>GSHMSQATSQPINFQVQKDGSSEKSAMDDYMQHPGKVIKQNNKYYFQTVLNNASFWKEYKFYNANNQELATTVVNDNKKADTRTINVAVEPGYKSLTT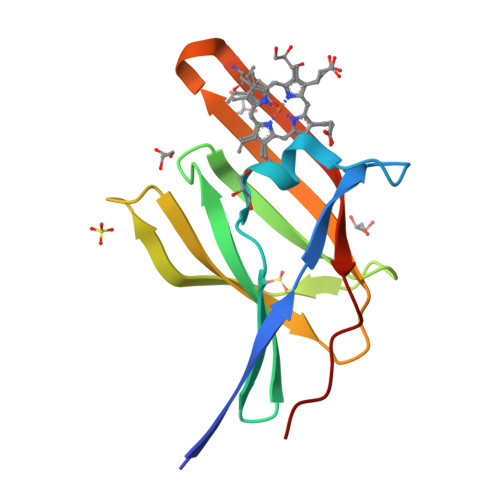KVHIVVPQINYNHRYTTHLEFEKAIPTLA[2x]> MRQCVVRRYKMPKNMGVAPRFDTWNEKYEPWEHMKRMGRLVGTGFYIPPEWYNHFRMFPPINHNFQQEKTLNPHNASEPTQDDTSTLSPERVALRDELARKSRLVASEGMRYYNIFWVRKPLDTMEKEYYELKRRGVDHGEAIRKVLQGFYS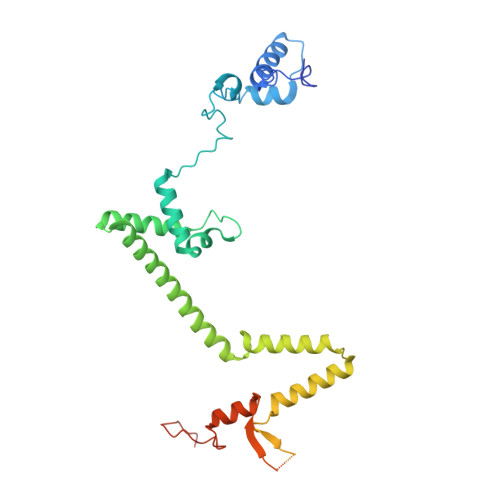GLAVKKRVAAIQAEEAKLTGRFITMREATVVLGVLAKLHKEQLTPHQVSLLAKEQGETTQSGAKLTAIVSRTQPHVNKEASSPATSEAVGSSTEESLSADALASMLSEDGEQSAVGTRYQVEVKETANDSVRQLREKAEDQTGFPDWYTGESPTYSGTSXCSRDGFALMKANK>MSHHHHHHSMDIEFMTEGPYKLPPGWRWVRLGEVCLPTERRDPTKNPSTYFVYVDISAIDSTVGKIVSPKEILGQHAPSRARKVIRSGDVIFATTRPYLKNIALVPPDLDGQICSTGFCVIRANREFAEPEFLFHLCRSDFITNQLTASKMRGTSYPAVTDNDVYNTLIPLPPLEEQRRIVAKVEALMERVREVRRLRAEAQKDTELLMQTALAEVFPHPGADLPPGWRWVRLGEVCDIIMGQSPPSSTYNFEGNGLPFFQGKADFGDLHPTPRIWCSAPQKVARPGDVLISVRAPVGSTNVANLACCIGRGLAALRPRDSLERFWLLYYLHYLEPELSKMGAGSTFNAITKKDLQNVFIPLPPLEEQRRIVAYLDQIQQQVAALKRAQAETEAELKRLEQAILDKAFRGDL[2x]

Restriction-modification (R-M) systems maintain the integrity of bacterial genomes by cleaving foreign DNA. Type I R-M enzymes are composed of three different subunits: a specificity subunit (HsdS or S) that recognizes specific DNA sequences, a methylation subunit (HsdM or M) that methylates target adenine bases, and a restriction subunit (HsdR or R) that translocates from the recognition site and cleaves DNA at variable positions. The HsdS subunit consists of two globular domains that correspond to the variable target recognition domains (TRD1 and TRD2) and two conserved regions (CR1 and CR2) that separate the TRDs. M2S1 is also the core DNA-binding component of the R-M enzyme. Together, the M2S1 complex recognizes an asymmetric, bipartite nucleotide target containing two specific regions 3 to 5 bp in length that are separated by nonspecific DNA sequences of 6 to 8 bp.

We report here the crystal structure of HsdS from Thermoanaerobacter tengcongensis in an open form conformation at 1.95 Å resolution. TRD1 and TRD2 exhibited very similar folds. In TTE-HsdS, the CRs were found to be composed of two long antiparallel α-helices, forming a coiled coils motif. The two helices were held together mainly by hydrophobic interactions and four hydrogen bonds. A three amino acid loop (Gln375–Glu377) is inserted in the CR2 α-helice. And there is a fifty degree bend in CR2. Although both TRD1 and TRD2 have similar folds in the three HsdS subunits, the overall domain orientation is quite different. Compared to the EcoKI-HsdS computational model, significant bending and twisting of the CRs in TTE-HsdS crystal structure enlarges the angle and distance between the TRDs and also shows a small range of rotation between the TRDs. In summary, the crystal structure of TTE-HsdS shows an open form domain-orientation. The potential open state model of the M2S1 complex was proposed based on the structure of TTE-HsdS.> NDNIELVDFQNIMFYGDAEVGDNQQPFTFILDTGSANLWV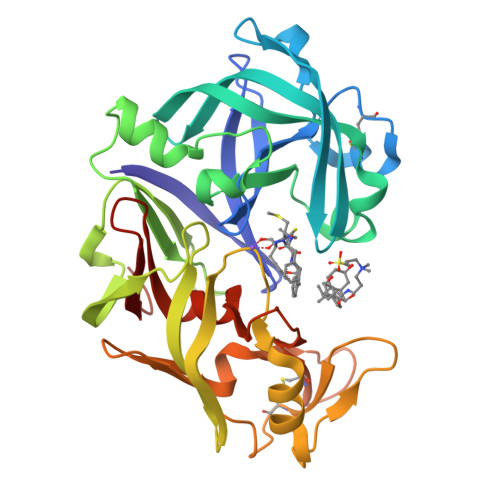PSVKCTTAGCLTKHLYDSSKSRTYEKDGTKVEMNYVSGTVSGFFSKDLVTVGNLSLPYKFIEVIDTNGFEPTYTASTFDGILGLGWKDLSIGSVDPIVVELKNQNKIENALFTFYLPVHDKHTGFLTIGGIEERFYEGPLTYEKLNHDLYWQITLDAHVGNIMLEKANCIVDSGTSAITVPTDFLNKMLQNLDVIKVPFLPFYVTLCNNSKLPTFEFTSENGKYTLEPEYYLQHIEDVGPGLCMLNIIGLDFPVPTFILGDPFMRKYFTVFDYDNQSVGIALAKKNL> MATPSFGNSSPQLTFTHVANFMNDAAADVSAVDAKQLAQIRQFLKANKTNLIESLNTIRQNVTSSGDHNKLRSTIANLLQINVDNDPFFAQSEDLSHAVEFFMSERSSRLHIVYSLLVNPDIDLETYSFIDNDRFNVVGKLISIISSVIQNYDIITASSLAHDYNNDQDMFTIVSLVQLKKFSDLKFILQILQILNLMILNTKVPVDIVNQWFLQYQNQFVEFCRNINSTDKSIDTSSLQLYKFQNFQDLSYLSETLISRISSLFTITTILILGLNTSIAQFDIQSPLYMDTETFDTVNSALENDVATNIVNEDPIFHPMIHYSWSFILYYRRALQSSESFDDSDITKFALFAESHDVLQKLNTLSEILSFDPVYTTVITVFLEFSLNFIPITASTSRVFAKIISKAPEQFIENFLTNDTFEKKLSIIKAKLPLLNESLIPLINLALIDTEFANFELKDICSFAVTKSSLNDLDYDLIADTITNSSSSSDIIVPDLIELKSDLLVAPPLENENSNCLLSIPKSTKGKILTIKQQQQQQQQQNGQQPPTTSNLIIFLYKFNGWSLVGRILQNLLHSYMEKGTQLDDLQHELMISIIKLVTNVVDPKTSIEKSSEILSYLSNSLDTSASTINGASIIQVIFEIFEISLQRKDYTSIVQCCEFMTMLTPNYLHLVSSYLNKSDLLDKYGKTGLSNMILGSV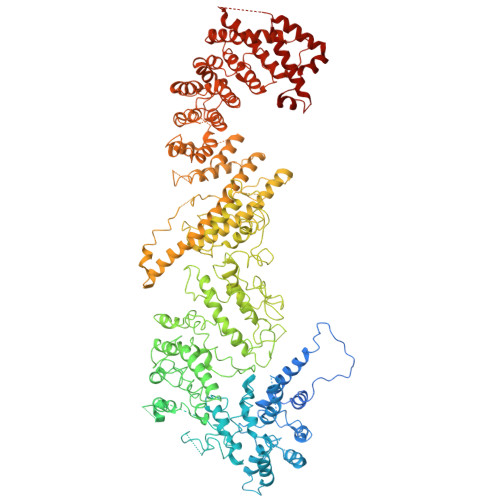ELSTGDYTFTIQLLKLTKVFIRESLSLKNIHISKRSKIDIINKLILHAIHIFESYYNWKYNNFLQKFEIAFHLTLIFYDVLHDVFTINPHQKDQLIISSSANKLLQLFLTPMDSIDLAPNTLTNILISPLNTTTKILGDKILGNLYSKVMNNSFKLCTLLIAIRGSNRDLKPSNLEKLLFINSSKLVDVYTLPSYVHFKVQIIELLSYLVEAPWNDDYPFLLSFLGEAKSMAFLKEVLSDLSSPVQDWNLLRSLYIFFTTLLESKQDGLSILFLTGQFASNKKINDESSIDKKSSILTVLQKNSLLLDSTPEEVSCKLLETITYVLNTWTNSKIFIKDPKFVNSLLAKLKDSKKLFQKKENLTRDETVSLIKKYKLISRIVEIFALCIYNSTDSNSEILNFLNQEDLFELVHHFFQIDGFNKTFHDELNLKFKEKWPSLELQSFQKIPLSRINENENFGYDIPLLDIVLKADRSWNEPSKSQTNFKEEITDASLNLQYVNYEISTAKAWGALITTFVKRSTVPLNDGFVDLVEHFLKLNIDFGSDKQMFTQIYLERIELSFYILYSFKLSGKLLKEEKIIELMNKIFTIFKSGEIDFIKNIGKSLKNNFYRPLLRSVLVLLELVSSGDRFIELISDQLLEFFELVFSKGVYLILSEILCQINKCSTRGLSTDHTTQIVNLEDNTQDLLLLLSLFKKITNVNPSKNFNVILASSLNEVGTLKVILNLYSSAHLIRINDEPILGQITLTFISELCSIEPIAAKLINSGLYSVLLESPLSVAIQQGDIKPEFSPRLHNIWSNGLLSIVLLLLSQFGIKVLPETCLFVSYFGKQIKSTIYNWGDNKLAVSSSLIKETNQLVLLQKMLNLLNYQELFIQPKNSDDQQEAVELVIGLDSEHDKKRLSAALSKFLTHPKYLNSRIIPTTLEEQQQLEDESSRLEFVKGISRDIKALQDSLFKDV1-[[(2R,3S,5S)-5-[5-methyl-2,4-bis(oxidanylidene)pyrimidin-1-yl]-3-oxidanyl-oxolan-2-yl]methyl]-3-(4-nitrophenyl)urea 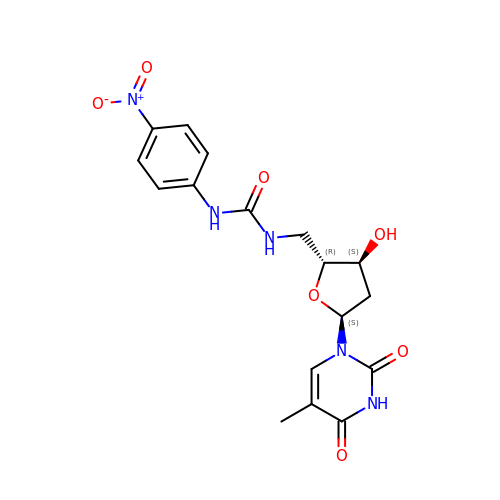| C17 H19 N5 O7 | GGXGAHUHZPSFRR-MJBXVCDLSA-N> KKVVARVAEARAEDVGK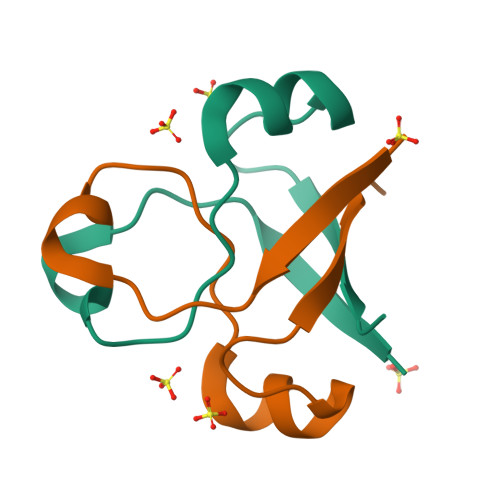RVVRVDKAERAKVGVKVGDVVEVKKV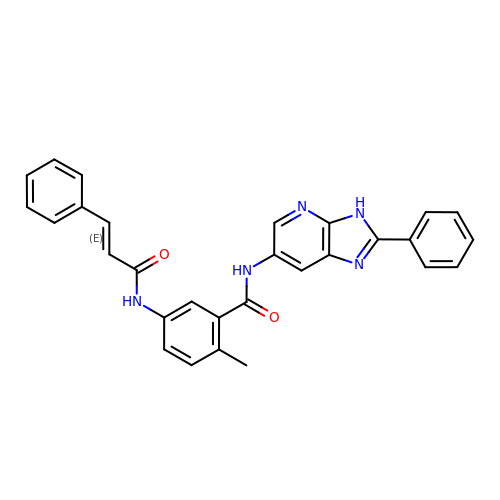2-methyl-N-(2-phenyl-3H-imidazo[4,5-b]pyridin-6-yl)-5-{[(2E)-3-phenylprop-2-enoyl]amino}benzamide | C29 H23 N5 O2 | ZNIFXENZPBLKBE-FYWRMAATSA-N>MRGSHHHHHHGSMVLGKPQTDPTLEWFLSHCHIHKYPSKSTLIHQGEKAETLYYIVKGSVAVLIKDEEGKEMILSYLNQGDFIGELGLFEEGQERSAWVRAKTACEVAEISYKKFRQLIQVNPDILMRLSAQMARRLQVTSEKLGNLAFLDVTGRIAQTLLNLAKQPDAMTHPDGMQIKITRQEIGQIVGCSRETVGRILKMLEDQNLISAHGKTIVVYGTR[2x]

CAP is a 210-amino-acid transcription factor that binds cAMP generated by adenylyl cyclase in response to the phosphorylated form of Enzyme IIAGlc (phosphorylated in response to the phosphoenolpyruvate-carbohydrate phosphotransferase system). cAMP-bound CAP regulates the transcription of over 100 genes crucial for carbon utilization through its binding to a specific promoter region and recruitment of RNA polymerase. Previous studies of the ligand binding domain of CAP demonstrated negative cooperativity between cAMP binding sites in the absence of structural change within this domain. We produce coarse-grained models that describe global low-frequency protein backbone motions of CAP and show a strong correlation between negative cooperativity for cAMP and modulation of the delocalised normal modes on ligand binding without a requirement for a spatially distinct physical pathway or conformational change. We demonstrate experimentally that altered connectivity between backbone elements in CAP can give predictable alterations to cooperativity for cAMP binding through altered mode amplitudes.

We examined amino acids predicted to show altered (V132, H160) or neutral (V140) responses to altered amino acid side chain interactions. The removal (V132A) or addition (V132L) of a side chain methyl group of V132 was engineered to decrease and increase, respectively, the strength of hydrophobic interaction across the dimer interface. Computation predicted that these mutations would result in more negative and positive cooperativity in CAP, respectively and that the most important contacts contributing to this effect were with L62 and V132 of the opposing monomer. High-resolution X-ray crystal structures of CAP mutants V132A and V132L demonstrated that these variants possessed decreased and increased hydrophobic interactions across the dimer interface, respectively. Comparison of variant crystal structures with wild-type demonstrated that there was no statistically significant change in structure. Cooperativity for cAMP binding was studied by isothermal titration calorimetry (ITC) for wild-type, V132A, and V132L proteins to examine whether the experimentally observed changes in cooperativity matched computational predictions. The qualitative computational prediction for altered cAMP cooperativity was tested experimentally including a significant controlled inversion of the sign of the cAMP cooperativity (V132L).>AQHNMRLQ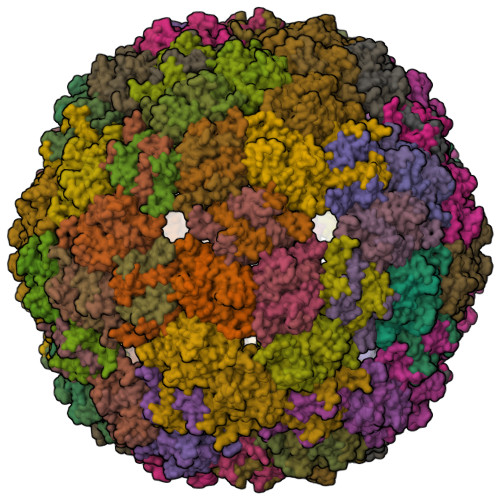LTSGTSLTWVDPNDFRSTFRINLNVNQKVAGAVSVYNARSEVITNRAPLVVIEGCTDACSVNRENISIRTTISGSVENKAAVLAALLDHLHNLGLARDDLVAGLLPTTIQPVVEYTGS[90x]>[2x]MELIRIAMKKDLENDNSLMNKWATVAGLKNPNPLYDFLNHDGKTFNEFSSIVNIVKSQYPDREYELMKDYCLNLDVKTKAARSALEYADANMFFEIEDVLIDSMISCSNMKSKEYGKVYKIHRELSNSVITEFEAVKRLGKLNIKTPEMNSFSRLLLLYHYLSTGNFSPMAQLIKQIDLSEISENMYIRNTYQTRVHVLMSNIKLNENSLEECREYSKKAL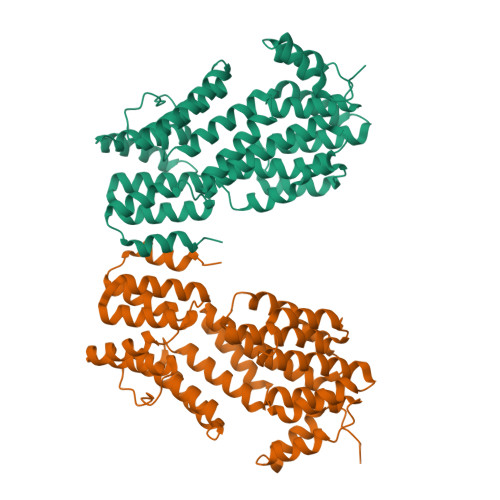ESTNILRFQVFSYLTIGNSLLFSNYELAQENFLKGLSISVQNENYNMIFQQALCFLNNVWRKENKWINFESDSIMDLQEQAHCFINFNENSKAKEVLDKLDLLVHNDNELAMHYYLKGRLEQNKACFYSSIEYFKKSNDKFLIRLPLLELQKMGENQKLLELLLLLEHHHHHHHH> MGIQVIATTPFKDQKPGTSGLRKPVPVFQQPHYLENFIQAIFDTIEAPQGQTLVLG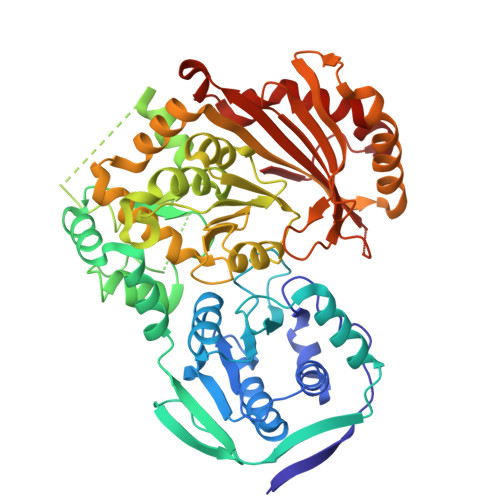GDGRYFNAEAIQVILKMAAAKGFARVKVGQNGILSTPAASCVIRKYGAVGGIILSASHNPAGPQGDFGVKFNIANGGPAPEKVTNAIYERSLALTHYSIYTAPDVNLHTLGEFPLGEMIVEVIDPVADYQALLETLFDFDRIAEVIRTGKLRLVFDAMHAVTGPYAQQILEKCLGAPPGTVQNGVPLPDFGGGHPDPNLVYAHDLVQQLFGEQPPDFGAASDGDGDRNMILGANCFVTPSDSLAILAANAQLVPGYRDGLAGIARSMPTSQAADRVAAKLGIDCYETPTGWKFFGNLLDAGKVTLCGEESFGTGSNHVREKDGLWAVLFWLNILAVRQTPVAEIVKDHWRTYGRNYYSRHDYEGIEGDRAHTLMSQLEQKLPSLVGQTLGAYTVATADNFSYSDPVDHSVSQNQGIRLIFEDGSRIVYRLSGTGTQGATLRVYLERFEPHPSQQHLDAQVALADLIQLANDVANIQSLTGRDRPTVIT YcjN is a putative substrate binding protein expressed from a cluster of genes involved in carbohydrate import and metabolism in Escherichia coli. YcjN is a poorly characterized putative SBP in Escherichia coli, whose protein-encoding gene is located within a cluster of 12 genes. In this cluster, three genes are predicted to encode protein components of an ABC transporter, including two TMDs (YcjO and YcjP) and an NBD (YcjV). Furthermore, previous studies using radioactive palmitate labeling have shown that YcjN is a lipoprotein.

We also report the first crystal structure of non-lipidated YcjN form (ΔYcjN) to a resolution of 1.95 Å. We chose the ΔYcjN protein for these crystallization studies because it does not aggregate in solution. The crystal structure was solved with P1 symmetry, and the asymmetric unit contained two molecules. The YcjN structure is composed of two α/β domains: the N-terminal domain (NTD) and the C-terminal domain (CTD) that can be divided into two subdomains (CTD1 and CTD2) (shown in teal, gray, and light blue, respectively). The NTD possesses a three-stranded β-sheet flanked by 11 α-helices (excluding linker segments). The CTD is composed of two subdomains (CTD1, residues 145–298 and residues 359–383; CTD2, residues 384–430) and is composed of three β-strands and 13 α-helices. The NTD and CTD are connected by three segments, including β7, β4, and α15. An analysis of the binding pocket revealed that there is no discernible electron density corresponding to a bound ligand deep within the binding pocket. However, a smaller electron density was detected at the edge of the binding pocket near tyrosine 95. SBPs that bind carbohydrates can also be members of subcluster B-I. However, these proteins lack the CTD2 domain, making them structurally distinct from subcluster D-I proteins. Due to YcjN’s molecular weight and the presence of the CTD2 domain, we group YcjN into subcluster D-I.

>[2x]MIKSKIVLLSALVSCALISGCKEENKTNVSIEFMHSSVEQERQAVISKLIARFEKENPGITVKQVPVEEDAYNTKVITLSRSGSLPEVIETSHDYAKVMDKEQLIDRKAVATVISNVGEGAFYDGVLRIVRTEDGSAWTGVPVSAWIGGIWYRKDVLAKAGLEEPKNWQQLLDVAQKLNDPANKKYGIALPTAESVLTEQSFSQFALSNQANVFNAEGKITLDTPEMMQALTYYRDLTANTMPGSNDIMEVKDAFMNGTAPMAIYSTYILPAVIKEGDPKNVGFVVPTEKNSAVYGMLTSLTITAGQKTEETEAAEKFVTFMEQADNIADWVMMSPGAALPVNKAVVTTATWKDNDVIKALGELPNQLIGELPNIQVFGAVGDKNFTRMGDVTGSGVVSSMVHNVTVGKADLSTTLQASQKKLDELIEQHHHHHHHHHHH> AEAAKPATAADSKAAFKNDDQKSAYALGASLGRYMENSLKEQEKLGIKLDKDQLIAGVQDAFADKSKLSDQEIEQTLQAFEARVKSSAQAKMEKDAADNEAKGKEYREKFAKEKGVKTSSTGLVYQVVEAGKGEAPKDSDTVVVNYKGTLIDGKEFDNSYTRGEPLSFRLDGVIPGWTEGLKNIKKGGKIKLVIPPELAYGKAGVPGIPPNSTLV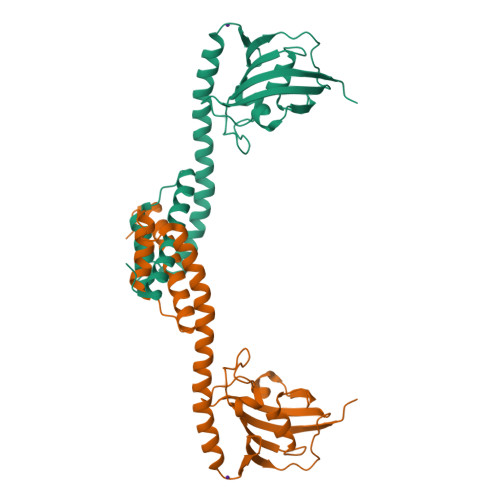FDVELLDVKPAPKADAKPEADAKAADSAKK> RSLPSCKEDEYPVGSECCPKCSPGYRVKEACGELTGTVCEPCPPGTYIAHLNGLSKCLQCQMCDPAMGLRASRNCSRTENAVCGCSPGHFCIVQDGDHCAACRAYATSSPGQRV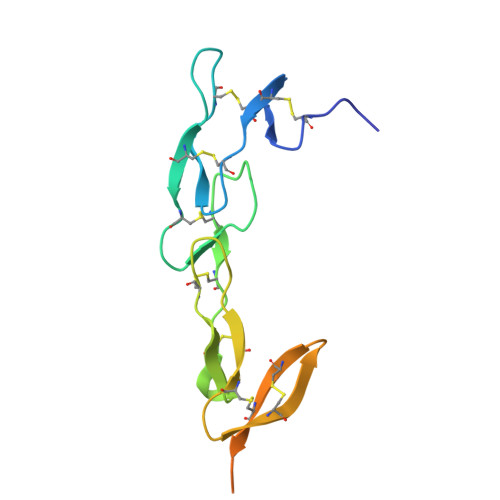QKGGTESQDTLCTGHHHHHH Tc toxins consist of three components: TcA, TcB, and TcC. The ~1.4 MDa TcA is a homo-pentameric bell-shaped molecule that mediates target cell association, membrane penetration, and toxin translocation. TcA is made up of a central, pre-formed channel that is enclosed by an outer shell composed of a structurally conserved α-helical domain decorated with variable receptor-binding domains (RBDs). Cryo-EM structures of Mm-TcdA4 and Xn-XptA1 in complex with heparin reveal that the glycan interacts with different parts of the shell domain, including receptor-binding domains.

We chose Mm-TcdA4 from the opportunistic human pathogen M. morganii to investigate the heparin/HS-toxin interaction in more detail. Since synthetic heparins/HSs are difficult to produce in the large amounts needed for biophysical and structural studies, we decided to work with natural ~15 kDa porcine intestinal mucosa heparin instead, regardless of its heterogeneity. We obtained BLI curves that show a rapid, concentration-dependent signal increase upon association and a signal decrease upon dissociation, indicating the tight interaction of Mm-TcdA4 and heparin. To identify which domains of Mm-TcdA4 are involved in heparin/HS binding, we determined the structure of Mm-TcdA4 in complex with porcine intestinal mucosa heparin using single particle cryo-EM. However, we identified additional densities at the periphery of the shell domain of each protomer. The density occupies a cleft that is predominantly formed by positively charged residues (R194, R195, K243, K265, R266, and R886), representing an ideal binding site for negatively charged heparins. This shows that unexpectedly heparins do not interact with an RBD or the neuraminidase-like domain at the tip of the shell, but directly with the α-helical domain of the shell. Although the resolution of the density does not allow to build an atomic model in this region, we flexibly fitted several heparin oligosaccharides that resemble natural heparin into the density. Indeed, most of them fit well and their negatively charged residues are involved in many potential electrostatic interactions at the interface. The heparin/HS binding site in the α-helical shell domain of Mm-TcdA4 is 10 nm away from the membrane if the Tc toxin is in the prepore conformation and attaches perpendicularly to the membrane.

>MDQITRILEKLNQQRSGETTVTLADFMPMSLAEIRSQNTGRLSREEAQLLHRAAQKEKQNNILYTARMLTRANPLLKKEMNTARYYGATPYGYDDIIPPRAEKFVAPGAVSSMFSPAGYLTELYREARGLHPKDSDRNLDKRRQDLAKLVLSQDNLDNEISALSLANEQLETALMAQTGKTDKNKYYETLATSRRSGVTPYNAPFEGIHNALAQRNFVLPDNILSNPAKFAILAAYDAGISPKLYNILTEDTESLTGSDLENSLKRNFPKVKIKDLMTLDALANYYELPADDIQALIAAEITGRLPTPDVYNDDNKLVIPAINTGGKITFSELAKTQSDEKQADYIDLIPQGGNQFLVNFSVKKTKKDATHFSIGYNKSFNNLADKNGFVPLAGEHYSIPVTLDAKILEKKTKIGITRKKPEPASDENHYTSATFTIHPNAEPGIWLLRLNKTLRLAKVSGMTPHETQHALIHVRNDSSEYELRRFTETLLYRKRYGIDTETALMLCNAGISRISYDGQLSHFDRLFNNPPLNGVTYTLGGDDILMEPDAGDPRREVLKRAFRVDNTGLWQLLVITNRENKSKTIENKTEKLRGLLFVRLLADVHNLTVAQLDALLQISPYNSMNVYALDGKTRQKMLSFLSRITQWLNTQNITVEQLMLLLDKISPAAPTKEMQVLLDLLRNGGIDKTNTKTLYTTMAPVITAAMQLDITESGEALLRWLDNNHPAGILTTSEARKLIIKKGQTAGDKEKLAAWCQALAQRVLVIRTFTLSNAELQTLSQGAPAGTITELYNISDFHNLINRCGEQAGTVLDALQSGTLTVKILAQALNLSEEVITQALTLAGQKPELTTWAQLAVLPPRLDLADTLHITPKDITTLLTVSENVRPFYTDLSALAGLLQAGLNEQQTKQLQNQSEPRRNEALSGEYRSLVMNNPVADRDDIWRNLLVDGKVSAEITTTLLADAIAGIQLYINRTIAGDEPGADSDALERQFFKDWDACNKRYSTWAGVSQLVYYPENFVDPTLRTGQTGMMNTMLEQLSQSELNKDTLENGFRQYLTAFEQVADLKVVSGYHDTVNINQGNTWFIGTSQTEPKKYYWRKADHSKCQNGRFAANAWSDWKEITCAVNPYGDMVRPVIFHSRLYLLWIEKQVQKDNTGKDTASFTLKLTHVKYDGSWASPFSYDITEKNISGWKKTGLYCAASQEDNSLLIAWYQIEKETQPNSFGLHIQPDMSCKKEPNIAGILATVTHQLDTETTVRVNTLLNRISSFEFTLEKQEGNKEIDLVISHGDYTVKTENSISALILNPTAYINITPYKLFSDIPDFYREKYITHLNSHSGTVYAPESKKMEPANNAISDKVNACAVYTYNNKPPKKHISLSIGKNYPLITPLELVGRKLESFFIKHKETSALYYTYGDATDDRLTLEEDKYTISTGEKKLGTLSLGKMIAQVKTISSDDISMEIELNSTKFETITGSDVGLRPPLYPTVSRETLAFPFGKLSITIPAGADINNLDCTIKVRFKNTDVLAATTTYKLVIKKTDPVQKVISLYTTPDGAQYMEWDGYRTRLNTLFTRQLIERANNGIDAILSPETQYLPEPKPGQGTYVTLILKPYDKNTHGTNRAFTIYYSNDATGSGKFPVYSGSLSVTDNTEVKLFIPLIKPGKNAVSQSAGAQQDTLYLNATYQKEATKQILLFRTDNNPEGWTLDKSVNNGTFAGLAENGVTGLLQSGEPMDFSGANALYFWELFYYTPMMVATRLLQEQNFTEANRWLSYIWQPAASGAGDWRVRPLKEDTSWNADPLDSVDPDAVAQNDPMHYKVSTLMKLLDLLIARGDKAYRMQERDTLNEAKMWYMQALGLLGDKPVSIFSNGWENPSLSNAADKTQAKQFHDEISRIRSGGLLPDVRTANTLTGLFRPQQNEKLLGYWQMLEMRLFNLRNNLSIDGQPLSLPVFAAPADPAALLSAAAAASGGSKPLPSADIPAMRFPQALDSARSLTGQLMQFGSTLLGLIERRDAEAMSELLQNQAGELMLSSLRMQEQALTELDAEKKILEQSRAGAQSRVDSYRALYDENVSAEEKRTMDLYLSSAILSTSIGVLDMAAAAADMAPNIFGVAVGGSRWGGIPKAIGAGMSLAASATKITADNISQSEAWRRRRQEWEIQKNNAESEIRQIDAQLEALAVRRTATEMQREHMEIQQAQTQAQLEFLQRKFSNKALYSWLRGRLASIYYRFYDLTAARCMMAEKAYAWQTNDTATRYIKSGAWQSNNAGLMAGESLLLNLAEMEQAWLKRDSRSLEVTRTVSLAAVYRTDNVTLAEGIADLLKGNGSGNIPASTGLSMTADNQLHAAFNLKALNIKDDYPEALGTTRRIKQISVTLPALVEPYQDMRAIFRYGGNSLPAGCKAIALSHGINDDGLFRLDFNDGRWLPFEGIPVDDDNSLTLSFPDATGEKQKPLLLSLTDIIIHIRYTIC[5x]12-methoxy-Nb-methylvoachalotine 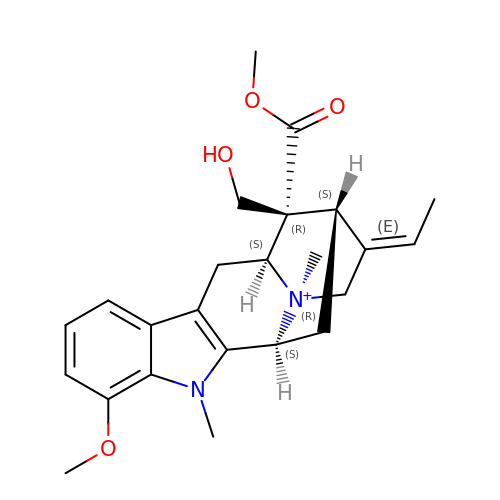| C24 H31 N2 O4 | LXYOQAOPFZZHKS-ROHZQTCMSA-N> NAKNKESPTKAIVRLREHINLLSKKQSHLRTQITNQENEARIFLTKGNKVMAKNALKKKKTIEQLLSKVEGTMESMEQQLFSIESANLNLETMRAMQEGAKAMKTIHSGLDIDKVDETMDEIREQVELGDEISDAISRP

The endosomal sorting complexes required for transport (ESCRTs) are membrane remodeling machinery that mediate diverse fundamental cellular processes, including the biogenesis of multivesicular body (MVB) during receptor down-regulation, enveloped virus budding, cytokinesis, plasma membrane repair, nuclear pore complex assembly, and nuclear envelope reformation. ESCRT-III is a unique protein complex in that it is metastable and conformationally dynamic, forming hetero-oligomeric filaments of multiple subunits on membranes. Vps20 nucleates the homo-oligomerization of the most abundant ESCRT-III subunit, Snf7, which then recruits Vps24 and Vps2. We then crystallized and solved X-ray crystal structures of Snf7core in two conformations at 1.6 Å and 2.4 Å resolutions, respectively.

By selectively removing its autoinhibitory C-terminus, we determine the first crystal structure of the Snf7 core domain in the active conformation at 1.6 Å resolution. Surprisingly, rather than adopting a rigid four-helix coiled-coil, the core domain undergoes a large-scale conformational rearrangement to extend into a highly elongated structure. This conformational change not only extends a cationic membrane-binding surface, but also exposes hydrophobic and electrostatic protein interacting surfaces for polymerization. Comparison of our Snf7core crystal structures we determined revealed two distinct conformations. Although both structures exhibit an open conformation, we noted two different orientations of α4 with respect to the α1/2 hairpin. In open conformation A, α4 extends in the protofilament plane, whereas in open conformation B, α4 is positioned perpendicular to the protofilament plane. Superimposing the two conformations revealed that α4 can rotate by at least ~90° along the axis of the α2/3 helix. Despite the large differences in α4 positioning, α4 makes a similar interaction with the α1/2 hairpin of a Snf7 protomer in a neighboring protofilament in both structures. This supports a model in which the assembly of the extended α2/3 helix upon Snf7 activation results in two key events: (1) α4 can no longer bind in cis to its own protomer; (2) α5 is displaced from the α1/2 hairpin.>[8x]SQKFGFIGLGIMGSAMAKNLVKAGCSVTIWNRSPEKAEELAALGAERAATPCEVVE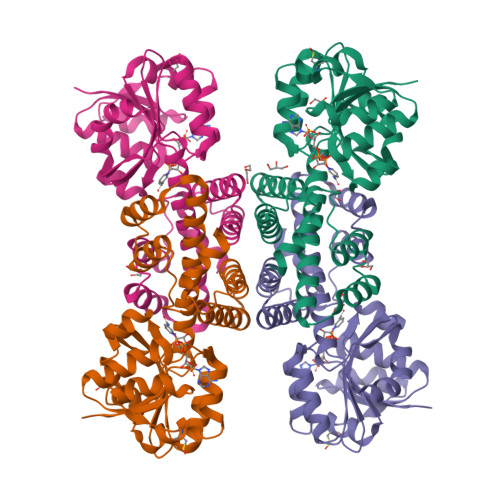SCPVTFAMLADPAAAEEVCFGKHGVLEGIGEGRGYVDMSTVDPATSQRIGVAVVAKGGRFLEAPVSGSKKPAEDGTLIILAAGDRNLYDEAMPGFEKMGKKIIHLGDVGKGAEMKLVVNMVMGGMMACFCEGLALGEKAGLATDAILDVIGAGAMANPMFALKGGLIRDRNFAPAFPLKHMQKDLRLAVALGDRVGQPLVASAAANELFKGARAAGFGDEDFSAIFKTYER>KPLPDYVAWKDADALIVHSDKTLETKRSEFGTSIITPEEKLYIQNNVNTPPESILADRDGWKVEISGVKEPRTLTVAELKTLGLVTAATVLQCSGNGRKYFKDQLTGDQKMSGTPWTVGAAGCVIWSGVPLKAVVDALGGPAEGARFITGTGGEELPAGLDPKLLVVERSVPISNLDNVILAWEMNGRPLSLAHGGPLRMVVPGYSGVNNIKYVKAVAMTEVETDAKIQKTSYRVHALGEKGSPDQPSVWEQPVKSWITTPHEAAKAGQVQIAGVAFGGMNACKSVEVSVDGGQTWQEAEF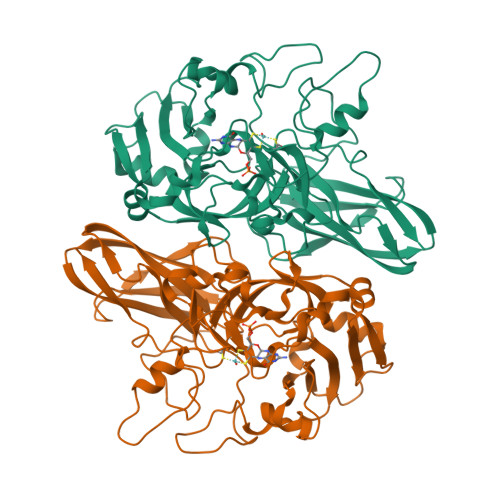IGPDLGRFAWRVFALSADLARGTYTLVSRATDTEGNVQPEETEMNGAGYGHNGWRAPAVKLTVA[4x]> MTSLIDLGRYVERTHHGEDTEPRSKRVKIAKPDLSSFQPGSIIKIRLQDFVTYTLTEFNLSPSLNMIIGPNGSGKSTFVCAVCLGLAGKPEYIGRSKKVEDFIKNGQDVSKIEITLKNSPNVTDIEYIDARDETIKITRIITRSKRRSDYLINDYQVSESVVKTLVAQLNIQLDNLCQFLSQERVEEFARLKSVKLLVETIRSIDASLLDVLDELRELQGNEQSLQKDLDFKKAKIVHLRQESDKLRKSVESLRDFQNKKGEIELHSQLLPYVKVKDHKEKLNIYKEEYERAKANLRAILKDKKPFANTKKTLENQVEELTEKCSLKTDEFLKAKEKINEIFEKLNTIRDEVIKKKNQNEYYRGRTKKLQATIISTKEDFLRSQEILAQTHLPEKSVFEDIDIKRKEIINKEGEIRDLISEIDAKANAINHEMRSIQRQAESKTKSLTTTDKIGILNQDQDLKEVRDAVLMVREHPEMKDKILEPPIMTVSAINAQFAAYLAQCVDYNTSKALTVVDSDSYKLFANPILDKFKVNLRELSSADTTPPVPAETVRDLGFEGYLSDFITGDKRVMKMLCQTSKIHTIPVSRRELTPAQIKKLITPRPNGKILFKRIIHGNRLVDIKQSAYGSKQVFPTDVSIKQTNFYQGSIMSNEQKIRIENEIINLKNEYNDRKSTLDALSNQKSGYRHELSELASKNDDINREAHQLNEIRKKYTMRKSTIETLREKLDQLKREARKDVSQKIKDIDDQIQQLLLKQRHLLSKMASSMKSLKNCQKELISTQILQFEAQNMDVSMNDVIGFFNEREADLKSQYEDKKKFVKEMRDTPEFQSWMREIRSYDQDTKEKLNKVAEKYEEEGNFNLSFVQDVLDKLESEIAMVNHDESAVTILDQVTAELRELEHTVPQQSKDLETIKAKLKEDHAVLEPKLDDIVSKISARFARLFNNVGSAGAVRLEKPKDYAEWKIEIMVKFRDNAPLKKLDSHTQSGGERAVSTVLYMIALQEFTSAPFRVVDEINQGMDSRNERIVHKAMVENACAENTSQYFLITPKLLTGLHYHEKMRIHCVMAGSWIPNPSEDPKMIHFGETSNYSFD;> MISTTISGKRPIEQVDDELLSLTAQQENEEQQQQRKRRRHQFAPMTQFNSNTLDEDSGFRSSSDVATADQDNFLEESPSGYIKKVILRNFMCHEHFELELGSRLNFIVGNNGSGKSAILTAITIGLGAKASETNRGSSLKDLIREGCYSAKIILHLDNSKYGAYQQGIFGNEIIVERIIKRDGPASFSLRSENGKEISNKKKDIQTVVDYFSVPVSNPMCFLSQDAARSFLTASTSQDKYSHFMKGTLLQEITENLLYASAIHDSAQENMALHLENLKSLKAEYEDAKKLLRELNQTSDLNERKMLLQAKSLWIDVAHNTDACKNLENEISGIQQKVDEVTEKIRNRQEKIERYTSDGTTIEAQIDAKVIYVNEKDSEHQNARELLRDVKSRFEKEKSNQAEAQSNIDQGRKKVDALNKTIAHLEEELTKEMGGDKDQMRQELEQLEKANEKLREVNNSLVVSLQDVKNEERDIQHERESELRTISRSIQNKKVELQNIAKGNDTFLMNFDRNMDRLLRTIEQRKNEFETPAIGPLGSLVTIRKGFEKWTRSIQRAISSSLNAFVVSNPKDNRLFRDIMRSCGIRSNIPIVTYCLSQFDYSKGRAHGNYPTIVDALEFSKPEIECLFVDLSRIERIVLIEDKNEARNFLQRNPVNVNMALSLRDRRSGFQLSGGYRLDTVTYQDKIRLKVNSSSDNGTQYLKDLIEQETKELQNIRDRYEEKLSEVRSRLKEIDGRLKSTKNEMRKTNFRMTELKMNVGKVVDTGILNSKINERKNQEQAIASYEAAKEELGLKIEQIAQEAQPIKEQYDSTKLALVEAQDELQQLKEDINSRQSKIQKYKDDTIYYEDKKKVYLENIKKIEVNVAALKEGIQRQIQNACAFCSKERIENVDLPDTQEEIKRELDKVSRMIQKAEKSLGLSQEEVIALFEKCRNKYKEGQKKYMEIDEALNRLHNSLKARDQNYKNAEKGTCFDADMDFRASLKVRKFSGNLSFIKDTKSLEIYILTTNDEKARNVDTLSGGEKSFSQMALLLATWKPMRSRIIALDEFDVFMDQVNRKIGTTLIVKKLKDIARTQTIIITPQDIGKIADIDSSGVSIHRMRDPERQNNSNFYN;> MGSVNSSPNEEFETVPDSQISGFDSPLIPTSVGSYFRDDDDDEKVHPNFISDPENDSLNSDEEFSSLENSDLNLSGAKAESGDDFDPILKRTIISKRKAPSNNEDEEIVKTPRKLVNYVPLKIFNLGDSFDDTITTTVAKLQDLKKEILDSPRSNKSIVITSNTVAKSELQKSIKFSGSIPEIYLDVVTKETISDKYKDWHFISKNCHYEQLMDLEMKDTAYSFLFGSSRSQGKVPEFVHLKCPSITNLLVLFGVNQEKCNSLKINYEKKENSRYDNLCTIFPVNKMLKFLMYFYSDDDNDDVREFFLKAFICLILDRKVFNAMESDHRLCFKVLELFNEAHFINSYFEIVDKNDFFLHYRLLQIFPHLQSALLRRRFSEKQGRTETIQQNIIKEFNEFFDCKNYKNLLYFILTMYGSKFIPFGPKCQVTEYFKDCILDISNETTNDVEISILKGILNLFSKIR;> MDGALINSVLYVSPRNGAHYFVELTEKHLLAFEMLNSMCLL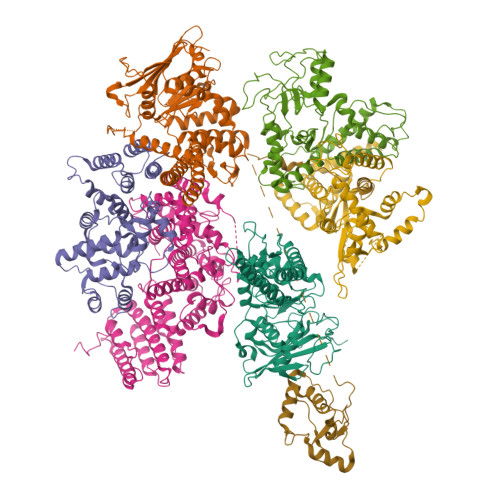ENYDHVLLFLECQFGKSHNLAVIPFDIILVLFTLSTLSEYYKEPILRANDPYNTSRETLSRRALKLLQKYLAILKEFDSEQYNLYDLELLRCQFFLAIDTLTPKKQKWGFDRFRRTKSESGVTYRQNASVDPELDQAKTFKNPYRSYISCLEQRNTILGNRLLNLKLNEPGEFINMILWTLSNSLQESTPLFLSSHEIWMPLLEILIDLFSCRQDYFIQHEVAQNVSKSLFVQRLSESPLAVFFESLNTRNFANRFSEYVFLNCDYKLPSDNYATPVHPVYNGENTIVDTYIPTIKCSPLYKSQKSLALRRKLIGSCFKLLLRVPDGHRLITPRIVADDVIQGISRTLASFNDILQFKKFFMTENLSQESYFIPLLAEGTLSEILKDTQECVVILTLVENLSDGVSFCNEVIGLVKSKCFAFTEQCSQASYEEAVLNIEKCDVCLLVLLRYLLHLIGTEAILDAKEQLEMLHAIEKNDSGRRQWAKALNLGNDPPLLYPIVSQMFGVHDKSVIIE;> MEVHEEQVSAPVTGDATAKYLLQYILSARGICHENALILALMRLETDASTLNTEWSIQQWVDKLNDYINAINVKLNLLGYKIIRINHGIGRNAVTLKAKQNFESFEDNTAIRAHNNDYAVLQSIVLPESNRFFVYVNLASTEETKLATRFNQNEIEFMKWAIEQFMISGETIVEGPALETSIIVKEVNRILVAATGDSNLAKWRKFSTFTVGSTNLFQFQELTATDIEDLLLRLCELKWFYRTQEGKFGIDLRCIAELEEYLTSMYNLNTCQNCHKLAIQGVRCGNESCREENEETGENSLSQIWHVDCFKHYITHVSKNCDRCGSSLITEGVYVI;> MSSIDNDSDVDLTEDLAVAKIVKENPVARKMVRYILSRGESQNSIITRNKLQSVIHEAAREENIAKPSFSKMFMDINAILYNVYGFELQGLPSKNNMNAGGNGSNSNTNKSMPEPLGHRAQKFILLNNVPHSKNFDDFKILQSAHTYEELIVTGEYIGDDIASGTSNTLESKLSTDRDLVYKGVLSVILCIVFFSKNNILHQELIKFLETFGIPSDGSKIAILNITIEDLIKSLEKREYIVRLEEKSDTDGEVISYRIGRRTQAELGLESLEKLVQEIMGLEKEQTKSLHDDIIKSIGDSYSI;> MSSTVISRKRRNSTVTEPDSSGETRKQKKSRSDEKSSSSKDGDPQLEFKVLQGYRDLESEMHKGRAQVTRTGDIGVAMDNLNAVDSLFNKVIGIKNNGLFAHDARAMVSISELAQISVRNLKFDDSRSMVNLENIVNSLKRYMLKEHFKLNNIAENRNDLTLAADEQSAADQQEESDGDIDRTPDDNHTDKATSSFKATSMRHSYLQQFSHYNEFSQFNWFRIGALYNTISKNAPITDHLMGPLSIEKKPRVLTQRRRNNDQVGEKITAEKITQHSLNSTQQETTPEQVKKCFKKLSKKLGPEGSINLFKFIIDPNSFSRSIENLFYTSFLIKEGKLLMEHDEEGLPTIKIKQSISHTDSRSKEIERQRRRAAHQNHIIFQMDMPTWRKLIKKYNITSPFLD> HHHHHEETLLNTKLETADLKWVTFPQVDGQWEELSGLDEEQHSVRTYEVCDVQRAPGQAHWLRTGWVPRRGAVHVYATLRFTMLECLSLP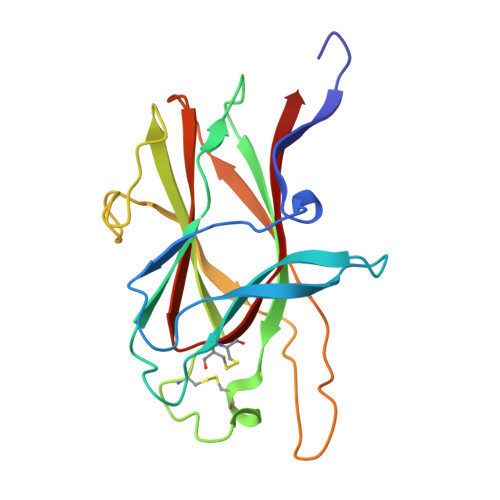RAGRSCKETFTVFYYESDADTATALTPAWMENPYIKVDTVAAEHLTRKRPGAEATGKVNVKTLRLGPLSKAGFYLAFQDQGACMALLSLHLFYKK>MSFANKQDPKTLVLFDVDGTLTPARLTISEEMKKTLEKLREKVVIGFVGGSDLSKQVEQLGPNVLNDFDYCFSENGLTAYKLGKELASQSFINWIGNEKYNKLVKFILRYLSDIDLPIRRGTFIEFRNGMINVSPIGRNASTQERNDYEKFDKQHHIRETMVEALKKEFPDFGLTYSIGGQISFDVFPTGWDKTYCLQHV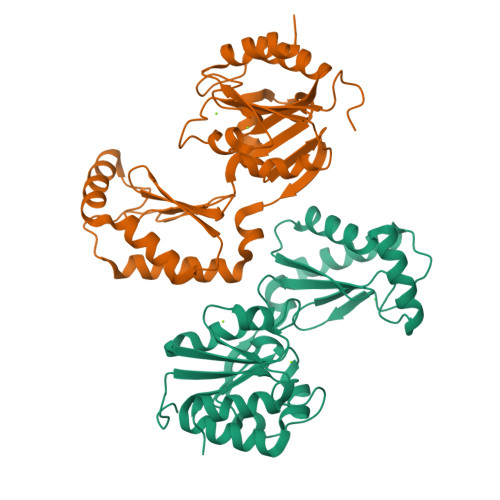EDEHFENIHFFGDKSYKGGNDYEIYNDPRTIGHAVNSPDDTIRILNETFKLQ[2x]>[4x]SLRVEETEVFKKYFKNLTDRER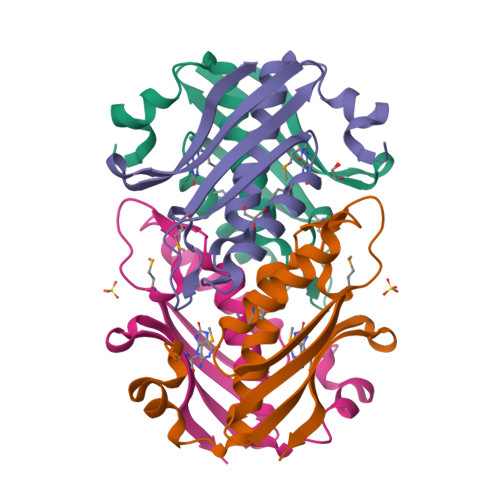AVFEGGITLGALFHQFVGTPVSKYNKESLERAIEEAMKNQPCVYDIKVKIRNVGEKYVSLDGKMLDVDLKIKINKTVAHLKLEYIPEIDYPLMYVKKFEE> MDVVSLDKPFMYFEEIDNELDYEPESANEVAKKLPYQGQLKLLLGELFFLSKLQRHG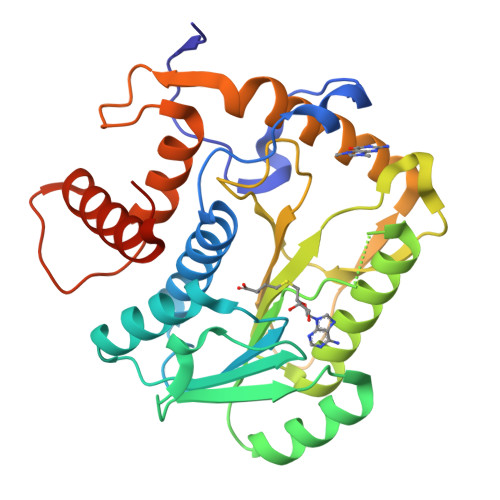ILDGATVVYIGSAPGTHIRYLRDHFYNLGVIIKWMLIDGRHHDPILNGLRDVTLVTRFVDEEYLRSIKKQLHPSKIILISDVRSKRGGNEPSTADLLSNYALQNVMISILNPVASSLKWRCPFPDQWIKDFYIPHGNKMLQPFAPSYSAEMRLLSIYTGENMRLTRVTKSDAVNYEKKMYYLNKIVRNKVVVNFDYPNQEYDYFHMYFMLRTVYCNKTFPTTKAKVLFLQQSIFRFLNIPTTSTEKVSHE2-(3,4-dihydroxyphenyl)ethyl beta-D-fructofuranoside | 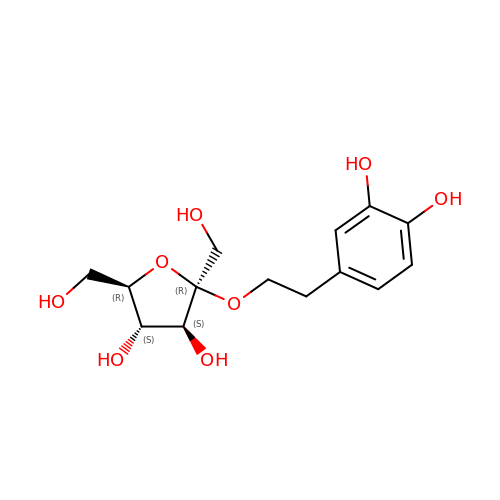C14 H20 O8 | LKYHMBCDFKCNAO-YIYPIFLZSA-N> SNARDPRPLRDKNFQSAIQEEIYDYLKKNKFDIETNHPISIKFLKQPTQKGFIIIFKWLYLRLDPGYGFTKSIENEIYQILKNLRYPFLESINKSQISAVGGSNWHKFLGMLHWMVRTNIKLDMCLNKVDRSLINQNTQEITILSQPLKTLDEQDQRQERYELMVEKLLIDYFTESYKSFLKLEDNYEPSMQELKLGFEKFVHIINTDVTSTELKLEELKVDLNRKRYKLHQQVIHVIDITSKFKINIQSSLENSENELGNVIEELRNLEFETEHNV;> SNASIFKDLEALSFQSNASRNQDVFPILDLQELVICLQSCDFALATQENISRPTSDYMVTLYKQIIENFMGISVESLLNSSNQETGDGHLQEENENIYLDTLNVLVLNKICFKFFENIGVQDFNMTDLYKPEAQRTQRLLSAVVNYARFREERMFDCNSFILQMESLLGQINKLNDEIKQLQKDFEVEVKEIEIEYSLLSGHINKYMNEMLEYMQ;> MSQKDNLLDNPVEFLKEVRESFDIQQDVDAMKRIRHDLDVIKEESEARLKLYRSLGVILDLENDQVLINRKNDGNIDILPLDNNLSDFYKTKYIWERLGK;> MASIDAFSDLERRMDGFQKDVAQVLARQQNHVALYERLLQLRVLPGASDVHDVRFVFGDDSRCWIEVAMHGDHVIGNSHPALDPKSRATLEHVLTVQGDLAAFLVVARDMLLASL;> EESYKRAAAVTSTLKARIEKMKAKSRREGTTRT

Ndc80 is part of a rod-like assembly, the Ndc80 complex, a heterotetramer composed of two coiled-coil heterodimers, joined end-to-end in parallel orientations. The globular domain at the N-terminal end of Ndc80:Nuf2 contacts microtubules; the globular domain at the C-terminal end of Spc24:Spc25 interacts, through two distinct adaptors, with the chromatin-proximal inner kinetochore. A further component of the response to erroneous attachment is the plus-end microtubule polymerase, Stu2 (the yeast ortholog of XMAP215/ch-TOG in metazoans). We describe experiments here in which we found that a C-terminal segment (CTS) of Stu2 bound specifically at the junction of the Ndc80:Nuf2 and Spc24:Spc25 heterodimers and that conserved features of the four-chain overlap at that junction were important for the interaction.

We instead used the ‘dwarf’ version of Ndc80c (Ndc80cdwarf) in which the coiled-coil shaft between the globular heads has been shortened to facilitate crystallization. We co-crystallized the Ndc80cdwarf with a 33-mer Stu2 peptide (Stu2 residues 855–888) and determined the structure of the complex by molecular replacement using the published Ndc80cdwarf structure as a search model. Clearly defined density in the resulting map corresponded to residues 862–888; there was no density corresponding to the N-terminal seven residues, and the C-terminal residues, 881–888, were part of a crystal-packing contact with the Nuf2 globular head of an Ndc80c symmetry mate. This lattice interaction may account for the somewhat different unit-cell dimensions in our crystals from those of the unliganded Ndc80cdwarf in the same space group, as well as for the nearly full occupancy but slightly higher local thermal parameters, as determined by refinement, for the low affinity peptide, which did not diffuse out during the short soak in cryopreservative. The peptide binds at the junction of the two heterodimeric subcomplexes, contributing a fifth α helix, and packs at about 30° to the main axis of the four overlapping helices from Ndc80, Nuf2, Spc24, and Spc25. Four conserved hydrophobic-residue side chains in the Stu2 CTS (V865, L869, I873, and M876) fit into hydrophobic pockets lined by conserved residues of Ndc80 and Spc24, and in a conserved polar contact, the side chain of Stu2 R872 inserts between D651 and S654 on Ndc80. As now shown here, the Stu2 CTS adds a fifth helix to the four-helix bundle, without producing any conformational rearrangements, indicating that the role of the junction is simply to anchor Stu2 along the Ndc80c rod, rather than to receive an allosteric signal from it. Fluorescence polarization binding experiments showed that the CTS binds dwarf Ndc80c with a dissociation constant of approximately 48 µM. The immobilized Ndc80cdwarf did not bind any mutant version of the Stu2 C-terminus.>[3x]ASMPAVERQLIECLHHVIKGAEPQQVGILCPQDDQRKALTEQFGSKTATSFCKEVDSLKNLSNLDALIVNQALDEEINDSEKLDKFITAALRSLRTDGVLILRQDLSKVKEMKKMAMLTD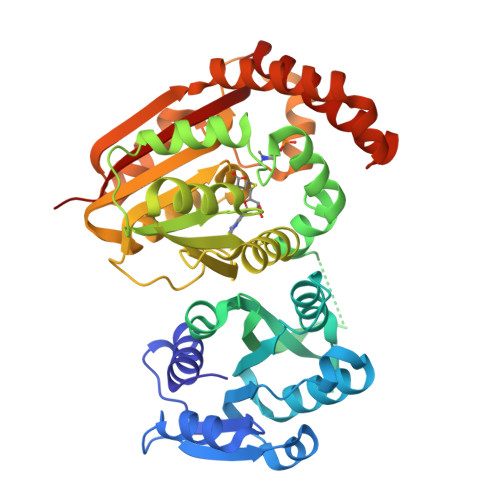YFDVFRLEEGNGNVGFQFYAVNEVLDSVYVHQNWLDFIWTLMKKPFPKDINGVVSFRDFLDRTQYTDTGIFAYEWIFGNNFISPGGWNQNLAILKRFGPMKTGQRMLDIGVGIGGGARQAASEFGLQVHGVDLSTNMLAVALERVHKEKDARVTYAVCDACEYEFEPNSFDYVFSRDCIQHIKDTDKLFSRIYRALKPGGKVLITMYGVGHGTLSESFKEYVSQRQYYLKNLEQIEEIAKKTGFIDIEVENMTPRFKEILLEERERIEQDKETFLAKFSQNAYDGLVSGWKSKLQYIADDNHNWNFFAAVKPQ>SMAMKATRLAIPDVILFEPRVFGDDRGFFFESYNQRAFEEACGHPVSFVQDNHSRSARGVLRGLHYQIRQAQGKLVRATLGEVFDVAVDLRRGSPTFGQWVGERLSAENKRQMWIPAGFAHGFVVLSEYAEFLYKTTDFWAPEHERCIVWN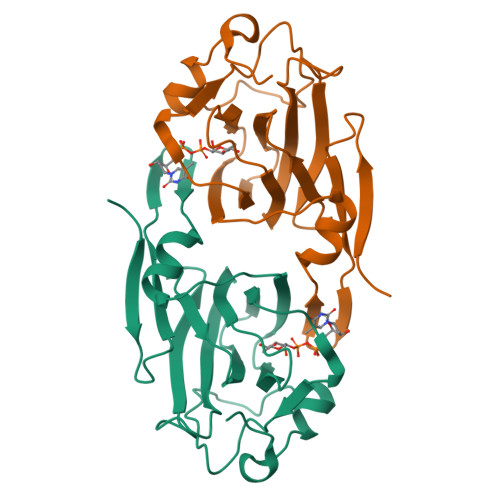DPELKIDWPLQDAPLLSEKDRQGKAFADADCFP[2x]>HGWVTDPPSRQALCASGETSFDCGQISYEPQSVEAPKGATTCSGGNEAFAILDDNSKPWPTTEIASTVDLTW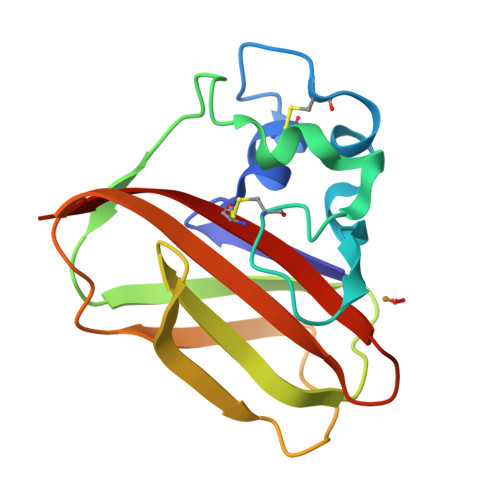KLTAPHNTSTWEYFVDGQLHQTFDQKGQQPPTSLTHTLTDLPTGEHTILARWNVSNTNNAFYNCMDVVVS[2x]>[2x]NPSNSDAAHAFWSTQPVPQTEDETEKIVFAGPMDEPKTVADIPEEPYPIASTFEWWTPNMEAADDIHAIYELLRDNYVEDDDSMFRFNYSEEFLQWALCPPNYIPDWHVAVRRKADKKLLAFIAGVPVTLRMGTPKYMKVKAQEKGEGEEAAKYDEPRHICEINFLCVHKQLREKRLAPILIKEATRRVNRTNVWQAVYTAGVLLPTPYASGQYFHRSLNPEKL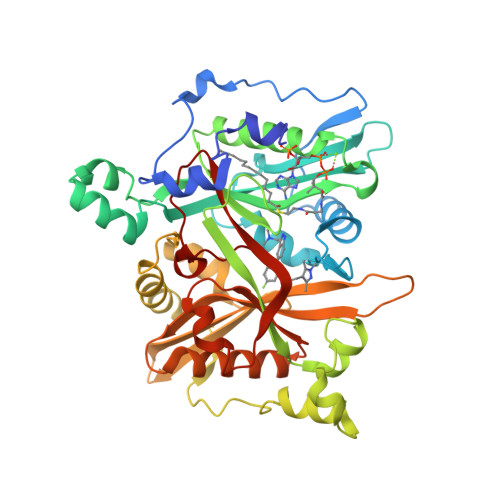VEIRFSGIPAQYQKFQNPMAMLKRNYQLPSAPKNSGLREMKPSDVPQVRRILMNYLDSFDVGPVFSDAEISHYLLPRDGVVFTYVVENDKKVTDFFSFYRIPSTVIGNSNYNLLNAAYVHYYAATSIPLHQLILDLLIVAHSRGFDVCNMVEILDNRSFVEQLKFGAGDGHLRYYFYNWAYPKIKPSQVALVML> CDDFLDRQVPQGIVTGDQIASPEYVDNLVISAYAIWATGDDINSSFSLWNYDVRSDDCYKGGSGTEDGGVFNALEISKGINTTDWNINDIWKRLYQCITRANTALQSLDQMDEKTYPLKNQRIAEMRFLRGHAHFMLKQLFKKIVIVNDENMEPDAYNELSNTTYTNDEQWQKIADDFQFAYDNLPEVQIEKGRPAQAAAAAYLAKTYLYKAYRQDGADNALTGINEEDLKQVVKYTDPLIMAKGGYGLETDYSMNFLPQYENGAESVWAIQYSINDGTYNGNLNWGMGLTTPQILGCCDFHKPSQNLVNAFKTDSQGKPLFSTYDNENYEVATDN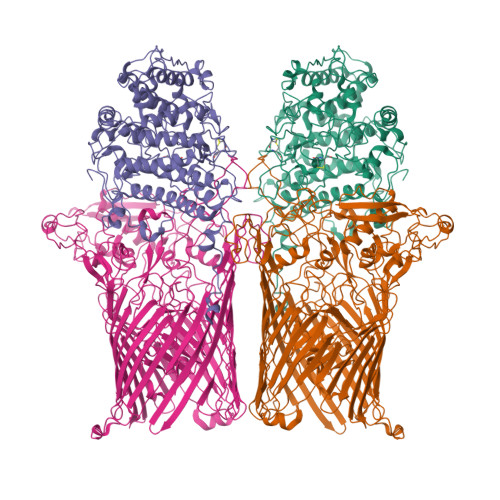VDPRLFHTVGMPGFPYKYNEGYIIQKNDDWSRSKGLYGYYVSLKENVDPDCDCLKKGSYWASSLNHIVIRYADVLLMRAEALIQLNDGRITDAISLINEVRSRAAGSTMLIFNYKEDYGVNFKVTPYDLKAYAQDEAMKMLKWERRVEFGMESSRFFDLVRWGEAKDVINAYYVTEASRCSIYKNAGFTENKNEYLPVPFEQISASNGNYTQNFGWAAAAHHHHHH;> VVVTGYTTQRKADLTGAVSVVKVDEIQKQGENNPVKALQGRVPGMNITADGNPSGSATVRIRGIGTLNNNDPLYIIDGVPTKAGMHELNGNDIESIQVLKDAASASIYGSRAANGVIIITTKQGKKGQIKINFDASVSASMYQSKMNVLNTEQYGRAMWQAYVNDGENPNGNALGYAYNWGYNADGNPVLYGMTLSKYLDSKNTMPVADTDWFDEITRTGVIQQYNLSVSNGSEKGSSFFSLGYYKNLGVIKDTDFDRFSARMNSDYKLIDDILTIGQHFTLNRTSEVQAPGGIIETALDIPSAIPVYASDGSWGGPVGGWPDRRNPRAVLEYNKDNRYTYWRMFGDAYVNLTPFKGFNLRSTFGLDYANKQARYFTYPYQEGTQTNNGKSAVEAKQEHWTKWMWNAIATYQLEVGKHRGDVMIGMELNREDDSHFSGYKEDFSILTPDYMWPDAGSGTAQAYGAGEGYSLVSFFGKMNYSYADRYLLSLTLRRDGSSRFGKNHRYATFPSVSLGWRITQENFMKELTWLDDLKLRASWGQTGNQEISNLARYTIYAPNYGTTDSFGGQSYGTAYDITGSNGGGVLPSGFKRNQIGNDNIKWETTTQTNVGIDFSLFKQSLYGSLEYYYKKATDILTEMAGVGVLGEGGSRWINSGAMKNQGFEFNLGYRNKTAFGLTYDLNGNISTYRNEILELPETVAANGKFGGNGVKSVVGHTYGAQVGYIADGIFKSQDEVDNHATQEGAAVGRIRYRDIDHNGVIDERDQNWIYDPTPSFSYGLNIYLEYKNFDLTMFWQGVQGVDIISDVKKKSDFWSASNVGFLNKGTRLLNAWSPTNPNSDIPALTRSDTNNEQRVSTYFVENGSFLKLRNIQLGYTVPAVISKKMRMDRLRFYCSAQNLLTIKSKNFTGEDPENPNFSYPIPVNITFGLNIGF>MEQAMRERSELARKGIARAKSVVALAYAGGVLFVAENPSRSLQKISELYDRVGFAAAGKFNEFDNLRRGGIQFADTRGYAYDRRDVTGRQLANVYAQTLGTIFTEQAKPYEVELCVAEVAHYGETKRPELYRITYDGSIADEPHFVVMGGTTEPIANALKESYAENASLTDALRIAVAALRAGSADTSGGDQPTLGVASLEVAVLDANRPRRAFRRITGSALQALLVDQESPQSDGESSG[14x];>TTIVALKYPGGVVMAGDRRSTQGNMISGRDVRKVYITDDYTATGIAGTAAVAVEFARLYAVELEHYEKLEGVPLTFAGKINRLAIMVRGNLAAAMQGLLALPLLAGYDIHASDPQSAGRIVSFDAAGGWNIEEEGYQAVGSGSLFAKSSMKKLYSQVTDGDSGLRVAVEALYDAADDDSATGGPDLVRGIFPTAVIIDADGAVDVPESRIAELARAIIESR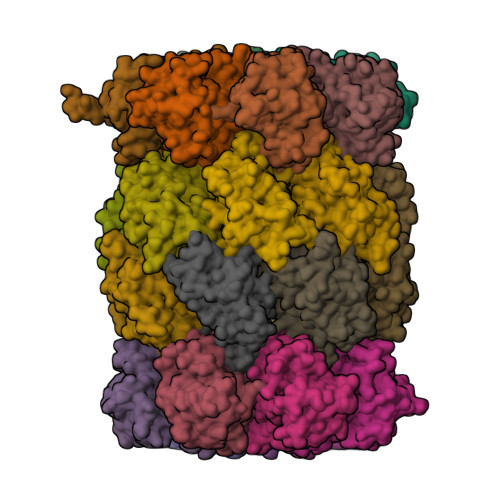SGADTFGSDGGEKHHHHHH[14x]>MPLLTIGDQFPAYQLTALIGGDLSKVDAKQPGDYFTTITSDEHPGKWRVVFFWPKDFTFVCPTEIAAFSKLNDEFEDRDAQILGVS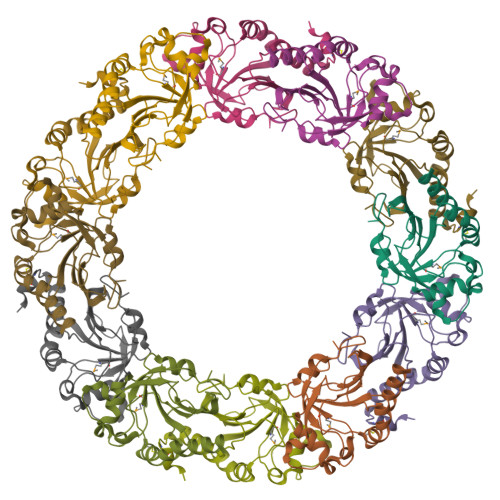IDSEFAHFQWRAQHNDLKTLPFPMLSDIKRELSQAAGVLNADGVADRVTFIVDPNNEIQFVSATAGSVGRNVDEVLRVLDALQSDELCASNWRKGDPTLDAGELLKASA[3x]>[2x]TLDGPYQPTSLNLPVD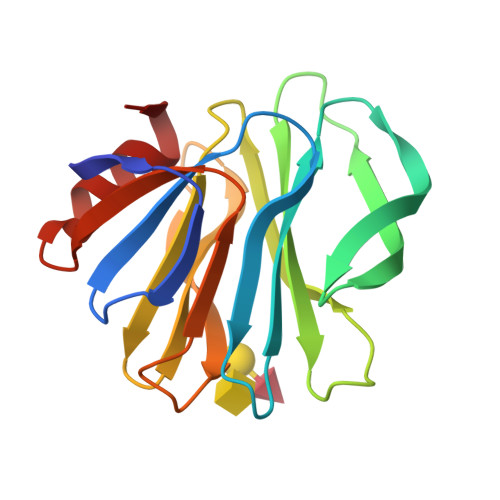YWMLIAPTREGKVAEGTNTTDRWFACVLVEPNVQNTQRQYVLDGQNVQLHVSNDSSTSWKFILFIKLTPDGTYTQYSTLSTPHKLCAWMKRDNRVYWYQGATPNASESYYLTINNDNSNVSSDAEFYLIPQSQTAMCTQYINNGL> XVNAKQYXRILKRRXARAKLX;> GPSFREQDIYLPIANVARIMKNAIPQTGKIAKDAKECVQECVSEFISFITSEASERCHQEKRKTINGEDILFAMSTLGFDSYVEPLKLYLQKFRE;> GPMEEIRNLTVKDFRVQELPLARIKKIMKLDEDVKMISAEAPVLFAKAAQIFITELTLRAWIHTEDNKRRTL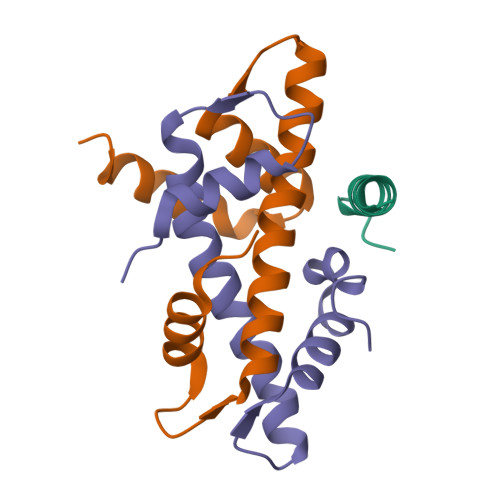QRNDIAMAITKFDQFDFLIDIVPR We characterized various features of the Salmonella-derived YfdX protein, including the crystal structure that contains a novel fold, previously unknown stoichiometric features, proof of contribution to antibiotic response, and participation in the control of bacterial virulence. Moreover, we found that Salmonella YfdX plays a significant role in bacterial susceptibility to penicillin G and carbenicillin and is involved in the negative regulation of bacterial virulence in an insect larvae model. Collectively, these data indicate that the recombinant st_YfdX protein can form a dimer or tetramer in solution, and this process is affected by pH of the solution. No homologous protein was identified in this search except for kp_YfdX (Z-score 20.1): a number of proteins containing a helical bundle were listed including Nitrosomonas europaea small metal-binding protein (Z-score 9.9) and E. coli cytochrome b562 (Z-score 8.5), but their structures overlapped with the st_YfdX structure only partially, indicating that YfdX adopts a novel protein fold that has not been identified yet.

Even though such a zinc coordination was not shown in our crystal structure, we did not exclude such a possibility completely, and thus attempted crystallization of the st_YfdX protein sample equilibrated with the final buffer consisting of 20 mM Bis-Tris-HCl (pH 6.0), 200 mM NaCl, 1 mM DTT, and 1 mM ZnCl2. Two forms of crystals were obtained that were diffracted to high resolution: rectangular crystals diffracted to 1.5 Å (space group F222; crystal II) under the same crystallization condition as that of crystal I, and board-shaped crystals diffracted to 2.3 Å (space group P222; crystal III) under the crystallization condition at pH 5.0. The asymmetric units of crystals II and III contain one and eight st_YfdX molecules, respectively. We once again determined the structure of st_YfdX using these crystals. Nevertheless, oligomerization-contributing zinc coordination demonstrated in the kp_YfdX structure (right) was not found in all our crystal structures of st_YfdX (not shown), indicating that the zinc coordination is not necessary for formation of the tetramer of this protein. Although both the tetrameric (at pH 7.5/8.0) and dimeric form (at pH 5.5/6.0) were confirmed by SEC-MALS and SAXS, st_YfdX was found to be in the tetrameric form in all the three crystal structures, presumably because of the increased opportunity of contacts in the crystal lattice.

>MAATNMTDNVTLNNDKISGQAWQAMRDIGMSRFELFNGRTQKAEQLAAQAEKLLNDDSTDWNLYVKSDKKAPVEGDHYIRINSSITVAEDYLPAGQKNDAINKANQKMKEGDKKGTIEALKLAGVSVIENQELIPLQQTRKDVTTALSLMNEGKYYQAGLLLKSAQDGIVVDSQSVQLEHHHHHH[8x]>[3x]MESRIWCLVVCVNLCIVCLGAAVSSSSTRGTSATHSHHSSHTTSAAHSRSGSVSQRVTSSQTVSHGVNETIYNTTLKYGDVVGVNTTKYPYRVCSMAQGTDLIRFERNIVCTSMKPINEDLDEGIMVVYKRNIVAHTFKVRVYQKVLTFRRSYAYIHTTYLLGSNTEYVAPPMWEIHHINSHSQCYS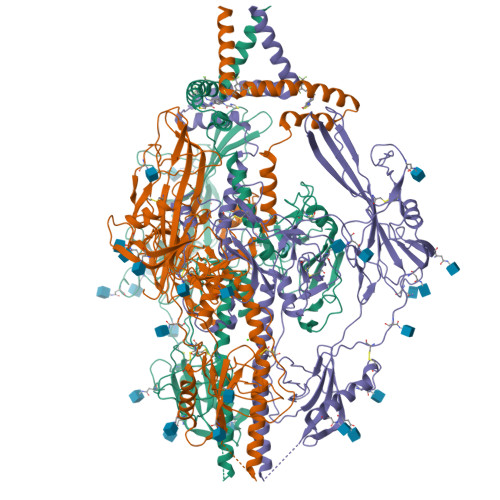SYSRVIAGTVFVAYHRDSYENKTMQLMPDDYSNTHSTRYVTVKDQWHSRGSTWLYRETCNLNCMVTITTARSKYPYHFFATSTGDVVDISPFYNGTNRNASYFGENADKFFIFPNYTIVSDFGRPNSALETHRLVAFLERADSVISWDIQDEKNVTCQLTFWEASERTIRSEAEDSYHFSSAKMTATFLSKKQEVNMSDSALDCVRDEAINKLQQIFNTSYNQTYEKYGNVSVFETTGGLVVFWQGIKQKSLVELERLANRSSLNLTHNRTKRSTDGNNATHLSNMESVHNLVYAQLQFTYDTLRGYINRALAQIAEAWCVDQRRTLEVFKELSKINPSAILSAIYNKPIAARFMGDVLGLASCVTINQTSVKVLRDMNVKESPGRCYSRPVVIFNFANSSYVQYGQLGEDNEILLGNHRTEECQLPSLKIFIAGNSAYEYVDYLFKRMIDLSSISTVDSMIALDIDPLENTDFRVLELYSQKELRSSNVFDLEEIMREFNSYKQRVKYVEDKVVDPLPPYLKGLDDLMSGLGAAGKAVGVAIGAVGGAVASVVEGVATFLKNPFGAFTIILVAIAVVIIIYLIYTRQRRLCMQPLQNLFPYLVSADGTTVTSGNTKDTSLQAPPSYEESVYNSGRKGPGPPSSDASTAAPPYTNEQAYQMLLALVRLDAEQRAQQNGTDSLDGQTGTQDKGQKPNLLDRLRHRKNGYRHLKDSDEEENV>[2x]ADPWQECMDYAVTLARQAGEVVCEAIKNEMNVMLKSSPVDLVTATDQKVEKMLISSIKEKYPSHSFIG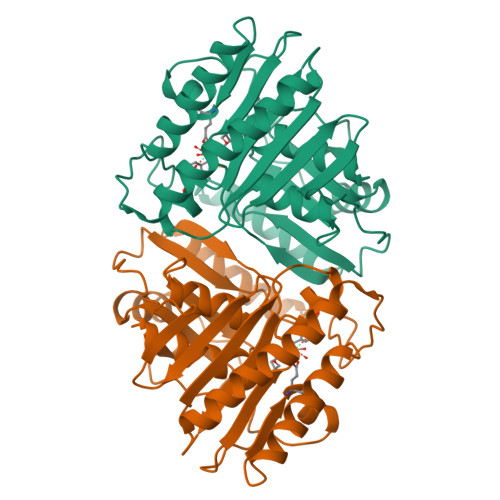EESVAAGEKSILTDNPTWIIDPIDGTTNFVHRFPFVAVSIGFAVNKKIEFGVVYSCVEGKMYTARKGKGAFCNGQKLQVSQQEDITKSLLVTELGSSRTPETVRMVLSNMEKLFCIPVHGIRSVGTAAVNMCLVATGGADAYYEMGIHCWDVAGAGIIVTEAGGVLMDVTGGPFDLMSRRVIAANNRILAERIAKEIQVIPLQRDDED> XT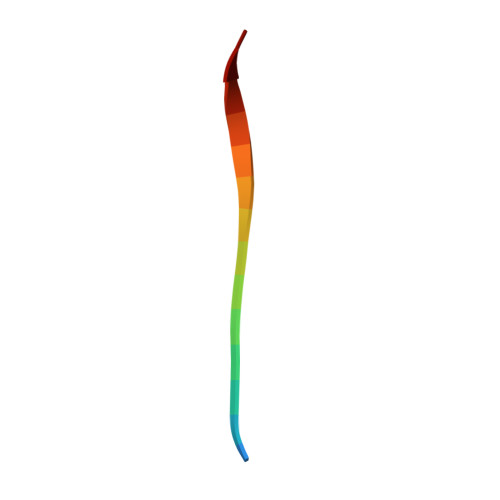EAAAGTGGVMTGR>[2x]MNTIAWLGRLVIERIRGIGVAALMLLQIIFSLPSAGGFGRFVYQMHRVGVMSLLIITVSGLFIGLVLGLQGYSILVNVGSESMLGTMVSLTLLRELAPVVAALLFAGRAGSALTAEIGSMKQSEQLASMEMIGVDPLKQIVSPRLWAGIVSLPMLTVIFAAIGIVGGKLVGVDFLGVDEGSFWSGMQNNVQFGHDVVNGIIKSIVFALLCTWIAVFQGYACDPTPEGIATAMTRTVVYSSLCVLGFDFVLTAVMFGGI;>[2x]MMNNKTPLSTQSLIEVKNLSFNRGERVIYDNISLNIRRGQITAIMGPSGTGKTTLLRLIGGQLVPDQGEVLLDGKDIAQMSRQELFAARARMGMLFQSGALFTDMSVYENVAFPIRAHTKLSENLIAELVALKLESVGLRGTEQLMPTELSGGMNRRVALARAIALDPDLIMYDEPFAGQDPIVKGVLTRLIRSLREALDLTTIIVSHDVPETLSIADYIYVVAEGKIQGEGTPEELQAYASPFVKQFLTGSAEGPVEYQFSHQAYLDNEVRP;>VVQYLNQELVVSGKIDFENAEQQYQAGLAIIKKQTSFPLIVDLKQLEHGNTLALAVLVQWLRQTPQKSGLHFKNVPEKMLKIIQACHLQEDLHLVLEHHHHHH[2x];>MKSRTSELAVGIFVIIFGIALFFLAMKVSGLVGTNLSDGYTMKAQFDNVNGLKPRAKVTMSGVTIGRVDSITLDPVTRLATVTFDLDGKLTSFNAEQLKEVQKNALDELRYSSDYTQATPAQQKTMEQQLISNMNSITSIDEDAYIMVATNGLLGEKYLKIVPGGGLNYLKRGDTISNTQGTMDLEDLISKFITGGGAGKVAAGSSSAEEKAPASTDSSAQPSFVE[6x]

The MlaFEDB complex is an ATP-binding cassette transporter to actively translocate the phospholipids between the inner membrane and the periplasmic protein MlaC4,5. The MlaFEDB-mediated glycerophospholipid (PL) transport was reported to play an important role in maintaining the integrity of the lipid membrane. Consistent with the previous reported low-resolution A. baumannii MlaFEDB map8 and our E. coli MlaFEDB map9 (EMD-30355), the MlaF (cytoplasmic nucleotide-binding domain, NBD), MlaE (transmembrane domain), MlaD (periplasmic phospholipid-binding domain), and MlaB (cytoplasmic auxiliary domain) subunits are assembled in a stoichiometry of 2:2:6:2. In summary, we characterize four structures of the A. baumannii MlaFEDB complex in nucleotide-free and vanadate-trapped conformations using single-particle cryo-EM.

The structure of MlaFEDB complex in nanodisc in nucleotide-free form was determined by cryogenic electron microscopy (cryo-EM). The final map of the MlaFEDB complex was well defined at 3.1 Å resolution, allowing us to build a nearly complete model for MlaFEDB, which includes a high-resolution structure of transmembrane helices (TMs) of MlaE and MlaD. The 3.1 Å resolution structure of nucleotide-free MlaFEDB reveals molecular details of the whole complex assembly and the glycerophospholipid binding, suggesting the unique and conserved features as compared to the E. coli MlaFEDB. Cryo-EM structure of MlaFEDB in nucleotide-free state also reveals glycerophospholipids bound inside the MlaE and MlaD, suggesting that the overexpressed A. baumannii MlaFEDB can bind glycerophospholipids from E. coli. Clusters of diacyl glycerophospholipid densities were resolved to be located in the central cavity and side cavities symmetrically. Two glycerophospholipids (PL center) are bound in the central cavity. Glycerophospholipid densities are also found on the two side cavities formed by MlaE and MlaD. The bound glycerophospholipids in the side cavity may play a role in the regulation of glycerophospholipid translocation or structural integrity of the complex. In the transmembrane region, the MlaFEDB complex consists of a total of 18 long helices in the inner membrane, formed by 2 subunits of MlaE and 6 subunits of MlaD. On the periplasmic side, the mammalian cell entry (MCE) domain of MlaD is assembled as a hexameric ring.>[2x]GGCGAUACCAGCCGAAAGGCC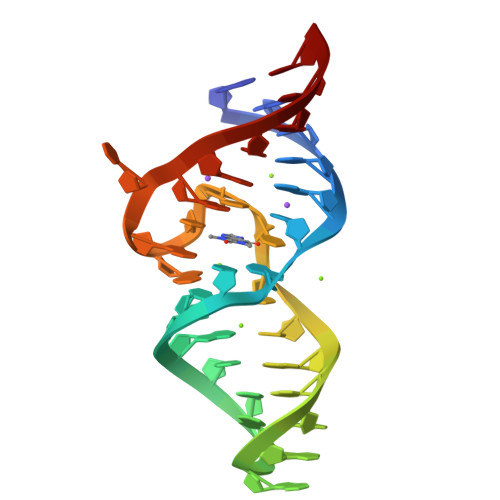CUUGGCAGCGCC> GAMGSTSLEPTSTLVRVRKSAATLGIAIEGGANTRQPLPRIVTIQRGGSAHNCGQLKVGHVILEVNGQTLRGKEHKEAARIIAEAFKTKERDYIDFLVTEFNVML;> 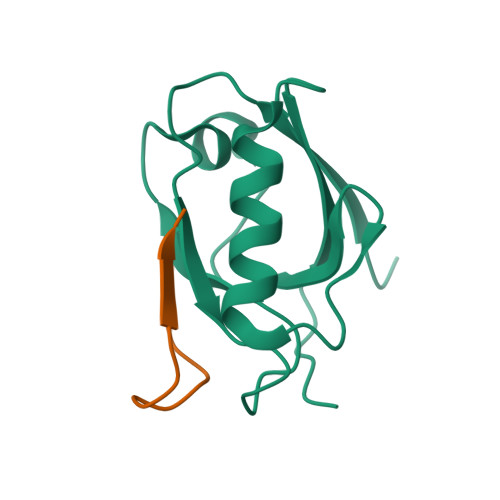ERLTLPPSEITLL> ASMTGGQQMGAPITAYAQQTRGLLGCIITSLTGRDKNQVEGEVQIVSTATQTFLATCINGVCWTVYHGAGTRTIASPKGPVIQMYTNVDQDLVGWPAPQGSRSLTPCTCGSSDLYLVTRHADVIPVRRRGDSRGS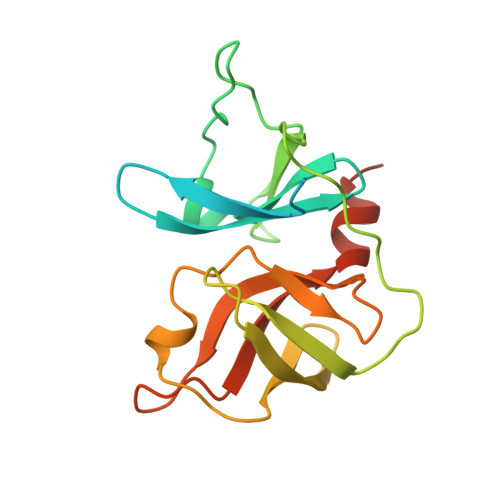LLSPRPISYLKGSSGGPLLCPTGHAVGLFRAAVCTRGVAKAVDFIPVENLETTMRGSHHHHHH6-[(3,5-dimethylphenyl)amino]-8-(methylamino)imidazo[1,2-b]pyridazine-3-carboxamide | C16 H18 N6 O | 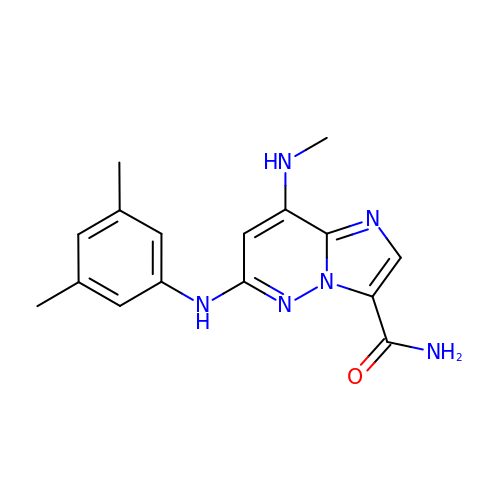SNVFFECYFQEWTL-UHFFFAOYSA-N> MGMVVALGLDFGTSGARAIACDFDSDRSVSVSVTFPKTSQNWPQVWREALWQLLTQIPADWRSRIERIAIDGTSGTVLLCDREGQPQTEPLLYNQACPIDLADLADWVPADHAALSSTSSLAKLWFWQQQFGALPPDWQILAQADWLSLQLHGCSQQSDYHNALKLGYSPDRERFSKNLLDSELGALLPVVHEPGVAIGPILPAIAQEFGLSPDCQICAGTTASIAAFLASGAHQPGEAVTSLGSTIVLKLLSQVAVSDRLTGVYSHKLGGYWLTGGASNCGGATLRQFFPDTELESLSCQIDPTKKSGLDYYPLPSRGERFPIADPDRLPQLEPRPENPVQFLQGLLEGLTQVETLGYQRLQDLGATPLKRIWTAGGGAKNAVWQQLRQQAIGVPIAIAPNTEAAFGTARLAAFGLAAFHSAGLKRTLEHHHHHH

Synpcc7942_2462 from the cyanobacteria Synechococcus elongatus PCC 7942 encodes a putative sugar kinase (SePSK), and this kinase contains 426 amino acids. The At2g21370 gene product from Arabidopsis thaliana, xylulose kinase-1 (AtXK-1), whose mature form contains 436 amino acids, is located in the chloroplast (ChloroP 1.1 Server). SePSK and AtXK-1 display a sequence identity of 44.9%, and belong to the ribulokinase-like carbohydrate kinases, a sub-family of FGGY family carbohydrate kinases. Domain I exhibits a ribonuclease H-like folding pattern, and is responsible for the substrate binding, while domain II possesses an actin-like ATPase domain that binds cofactor ATP.

Our results suggested that three conserved residues (D8, T11 and D221 of SePSK) play an important role in SePSK function. To identify the function of these three residues of SePSK, we constructed D8A, T11A and D221A mutants. Using enzymatic activity assays, we found that all of these mutants exhibit much lower activity of ATP hydrolysis after adding D-ribulose than that of wild type, indicating the possibility that these three residues are involved in the catalytic process of phosphorylation D-ribulose and are vital for the function of SePSK. The O4 and O5 of RBL1 are coordinated with the side chain carboxyl group of Asp221. Three conserved residues in SePSK were identified to be essential for this function.Here we describe extendable linear, curved and angled protein building blocks, as well as inter-block interactions, that conform to specified geometric standards; assemblies designed using these blocks inherit their extendability and regular interaction surfaces, enabling them to be expanded or contracted by varying the number of modules, and reinforced with secondary struts. We construct twistless helix repeat (THR) protein blocks from identical straight α-helices (typically 2–4 helices in each unit); the length of the blocks can be varied simply by varying the number of repeat units. Restricting helical geometry to ideal straight helices with zero helical twist in principle considerably limits what types of structure could be built, but this is more than compensated by the great simplification of downstream material design, as illustrated below. Using X-ray crystallography and electron microscopy, we validate nanomaterial designs ranging from simple polygonal and circular oligomers that can be concentrically nested, up to large polyhedral nanocages and unbounded straight ‘train track’ assemblies with reconfigurable sizes and geometries that can be readily blueprinted.

Expandability over four different sizes was achieved with cage_O43_129 (+0, +4, +8 and +12 helices). The internal structure of the oligomers is clearly resolved in cryo-EM reconstructions for the first three sizes and in ns-EM reconstruction of the largest size; the distance between the centre of mass of the tetramer component to the centre of mass of the trimer component across the different sizes is 7.9, 9.4, 11.3 and 11.7 nm respectively. Views down each of the three symmetry axes (twofold, threefold and fourfold) are clear for each size (except for the threefold view in the largest size) with slight rotational deviations of the fourfold cyclic component compared to the design model, whereas the rotation of the threefold cyclic component holding the THR remains unperturbed as designed.

>MGDDLLLKLLELLVEQARVSAEFARRQGDEKMLEEVARKAEEVARKAESIARKARKEGNLELALKALEILVRAAHVLAEIARERGNEELQKKAHKLAKEALRQVIEIAIRAIQEGNLELAIIALHISVRIAEVLLETRPDDREEIREQQAIFELLIAALEAAIRLEKLKEEGAPPEQIERVAEHGLERLKEIAKEISKEVDSPESKRIAYKIVAAAAEFLLKILAEGGATPEQLERVTEHALEVLKEVAKELADSPESGLAALAAIASLAKLGLEQLKEIGAPPEQQRRVTKAGIEAVREIYRYGRKLY[24x];>[24x]MGCDAIQAAAALGEAGISSNEILELLAAAAELGLDPDAIQAAAQLGEAGISSEEIKELLRAAHELGLDPDAIAAAADLGQAGVSPVEILALLIAASVLGLDPDAIQAAAALGEAGISAEEIIELLTAARDLGLDPDAIQAAAQLGEAGISSEEIKELLRAAHELGLDPDCIAAAADLGQAGISSSEITALLLAAAAIELAKRADDKDVREIVRDALELASRSTNDEVIRLALEAAVLAARSTDSDVLEIVKDALELAKQSTNEEVIKLALKAAVLAAKSTDEEVLEEVKEALRRAKESTDEEEIKEELRKAVEEAEGGSWLEHHHHHH>GSMPAVASVPKELYLSSSLKDLNKKTEVKPEKISTKSY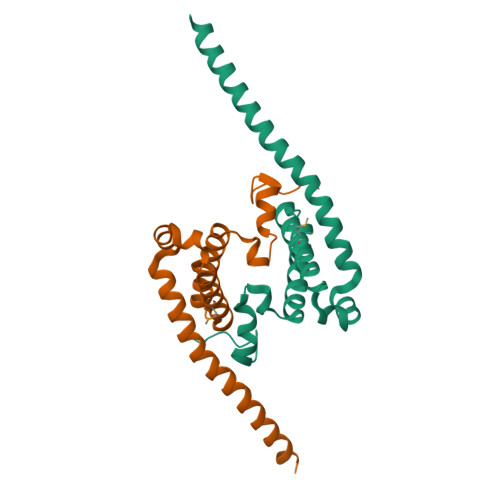VHSALKIFKTAEECRLDRDEERAYVLYMKYVTVYNLIKKRPDFKQQQDYFHSILGPGNIKKAVEEAERLSESLKLRYEEAEVRKKLEEKDRQEEAQRLQQKRQETG[2x]ACETOHYDROXAMIC ACID 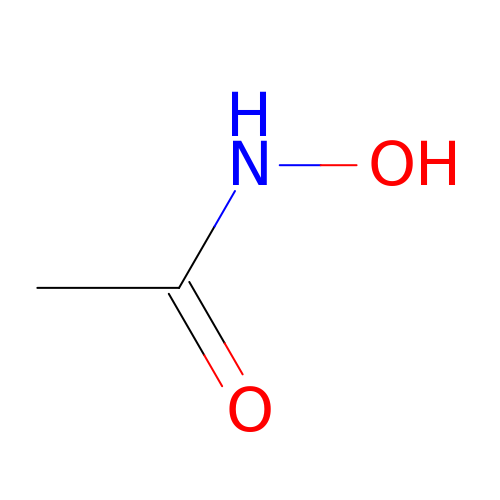| C2 H5 N O2 | RRUDCFGSUDOHDG-UHFFFAOYSA-N> MIVIFVDFDYFFAQVEEVLNPQYKGKPLVVSVYSGRTKTSGAVATANYEARKLGVKAGMPIIKAMQIAPSAIYVPMRKPIYEAFSNRIMNLLNKHADKIEVASIDEAYLDVTNKVEGNFENGIELARKIKQEILEKEKITVTVGVAPNKILAKIIADKSKPNGLGVIRPTEV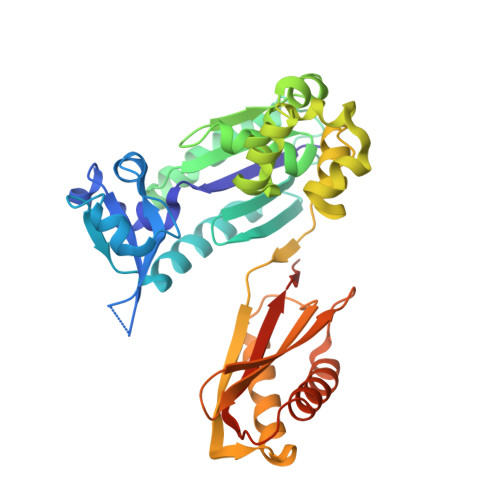QDFLNELDIDEIPGIGSVLARRLNELGIQKLRDILSKNYNELEKITGKAKALYLLKLAQNKYSEPVENKSKIPHGRYLTLPYNTRDVKVILPYLKKAINEAYNKVNGIPMRITVIAIMEDLDILSKGKKFKHGISIDNAYKVAEDLLRELLVRDKRRNVRRIGVKLDNIIINKTNLSDFFDI> ANDSIFFSPLKYLGAEQQRSIDASRSLLDNLIPPSLPQYDNLAGKLARRAVLTSKKLVYVWTENFANVKGVPMARSVPLGELPNVDWLLKTAGVIVELIVNFVASLPASAAAQFERIAAGLSGDLEAARQVHEALLEEAKNDPAAAGSLLLRFTELQTRVIALLTRVGLLVDDILKSASNLVTQGGQGDGLNRFRAVFGTLRLPEVADSFRDDEAFAYWRVAGPNPLLIRRVDALPANF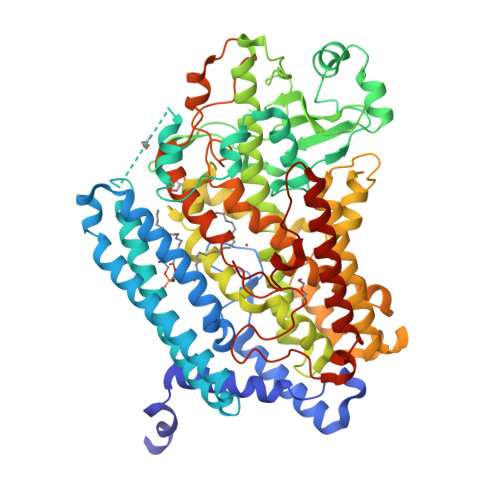PLGEEQFRRVMGADDSLLEAAASRRLYLLDYAELGKLAPSGAVDKLLTGTGFAYAPIALFALGKDRAGLLPVAIQCGQDPATHPMFVRPAESESDLYWGWQMAKTVVQVAEENYHEMFVHLAQTHLVSEAFCLATQRTLAPSHPLHVLLAPHFEGTLFINEGGARILLPSAGFIDVMFAAPIQDTQATAGGNRLGFDFYRGMLPESLKARNVDDPAALPDYPYRDDGLLVWNAIRQWAADYVAVYYASDGDVTADVELAAWVGEVIGSGKVAGFRPITGRSQLVEVLTMVIFTASAQHAAVNFPQPSMMTYAPAICAMSAAPAPDSPSGKSEADWLKMMPPTLVALEKVNIYHLLGSVYHGRLGDYRQTGFPYAPVFSDRRVTASGGPLERFQARLKEVEATIRTRNQARRKPYEYLLPSRIPASTNI>MSLIDPRAIIDPSARLAADVQVGPWSIVGAEVEIGEGTVIGPHVVLK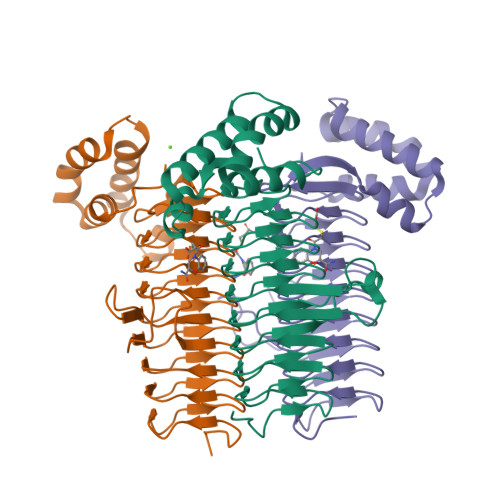GPTKIGKHNRIYQFSSVGEDTPDLKYKGEPTRLVIGDHNVIREGVTIHRGTVQDRAETTIGDHNLIMAYAHIGHDSVIGNHCILVNNTALAGHVHVDDWAILSGYTLVHQYCRIGAHSFSGMGSAIGKDVPAYVTVFGNPAEARSMNFEGMRRRGFSSEAIHALRRAYKVVYRQGHTVEEALAELAESAAQFPEVAVFRDSIQSATRGITR[6x]> VTLLD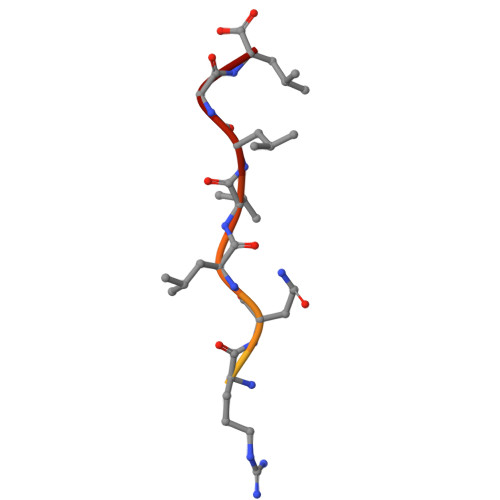PQMERQLVLGL>[8x]MIIKNYS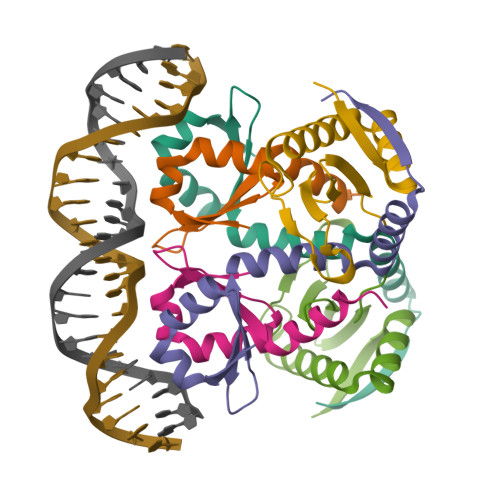YARQNLKALMTKVNDDSDMVTVTSTDDKNVVIMSESDYNSMMETLYLQQNPNNAEHLAQSIADLERGKTITKDIDV;>[4x]MARLNITFSPQAFEDYKYFQQNDKKMVKKINELLKSIDRNGALEGIGKPEKLKSNLTGYYSRRINHEHRLVYTVDDNHIKIASCKYHY>NTGLLESQLSRHDQMLSVHDIRLADMDLRFQVLETASYNGVLIWKIRDYKRRKQEAVMGKTLSLYSQPFYTGYFGYKMCARVYLNGDGMGKGTHLSLFFVIMRGEYDALLPWPFKQKVTLMLMDQGSSRRHLGDAF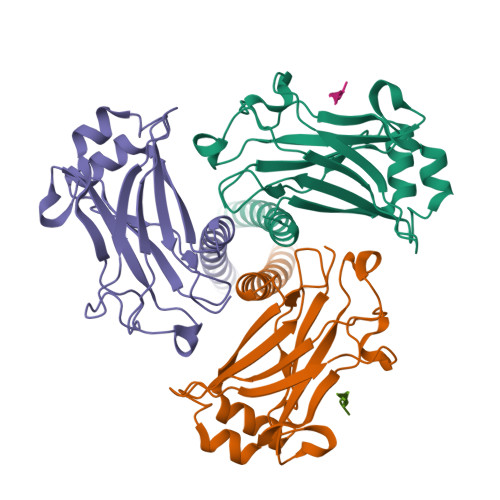KPDPNSSSFKKPTGEMNIASGCPVFVAQTVLENGTYIKDDTIFIKVIVDTSDLPDP[6x];>[3x]PIQAS> ELQKSIGHKPEPTDEEWELIKTVTEAHVATNAQGSHWKQKRKFLPEDIGQAPIVNAPEGGKVDLEAFSHFTKIITPAITRVVDFAKKLPMFCELPCEDQIILLKGCCMEIMSLRAAVRYDPESETLTLNGEMAVTRGQLKNGGLGVVSDAIFDLGMSLSSFNLDDTEVALLQAVLLMSSDRPGLACVERIEKYQDSFLLAFEHYINYRKHHVTHFWPKLLMKVTDLRMIGACHASR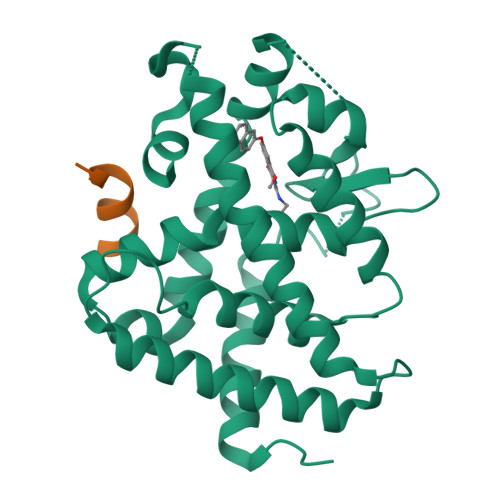FLHMKVECPTELFPPLFLEVFED;> ENALLRYLLDKD> MPARRPFIGGNFKCNGSLDFIKSHVAAIAAHKIPDSVDVVIAPSA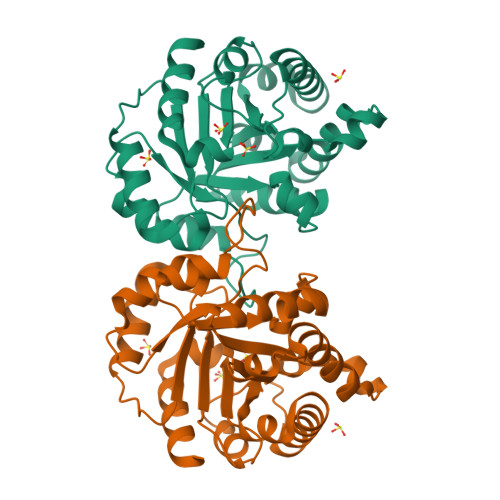VHLSTAIAANTSKQLRIAAQNVYLEGNGAWTGETSVEMLQDMGLKHVIVGHSERRRIMGETDEQSAKKAKRALEKGMTVIFCVGETLDERKANRTMEVNIAQLEALGKELGESKMLWKEVVIAYEPVWSIGTGVVATPEQAEEVHVGLRKWFVEKVAAEGAQHIRIIYGGSANGSNCEKLGQCPNIDGFLVGGASLKPEFMTMIDILTKTRT> MVIVPEGTQLDEKQHIVINNGAEPQSFDPHKTEGVPESNVAYQLLEGLVTSDSEGKLQPGAAESWENTPDFKTWTFHLRKDAKWSNGDPVTAHDFVFAWRRLVDPATAAPYASYLSYLQVENAQDIIDGKKKPAELGVEAKDDYTFVVHATNPVPYAVSLTTHQSLLPLPQKVVEKLGDAWVKKENYVGNGAYKLANHIINEKIEFERNPLYWNDKETVINSATFLAIENPSTDVARYRAGDLDMTSYGLPPEQFAKLKKELLGEVYVTRTLGTYSYELNNKKAPFDNVNIRKALNLSLDRNVITDKVLGQGQTPTYVFTPTYIEEGHLIQQPAYSKEPMAQRNEEAIKLLEEAGYSKANPLKFSILYNTNENHKKVA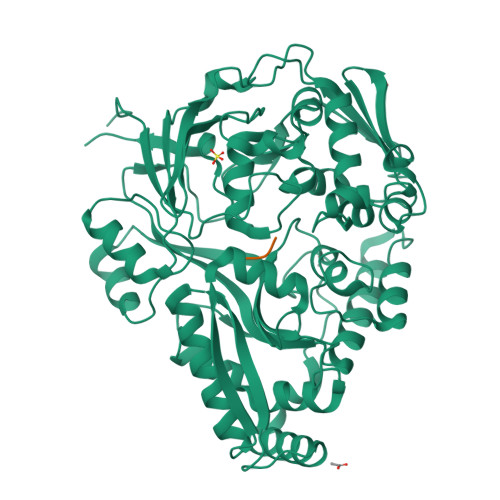IAAASMWKANTKGLIDVKLENQEWKTYIDSRRAGRYDVARAGWHADYNQATTFGNYFLSNSSNNTAKYANPEYDKAMAESYAATDAEGRAKAYAKAEEILGKDYGIVPIFNYVNPRLVKPYVKGYSGKDPQDHIYLRNLYIIKHLEHHHHHH;> MGG>MNSQQNPDLAVHPLAIPMEGLLGESATTLEKNVIATQLSEEAQVKLEVIQSLLEPCDRTTYGQKLREAAEKLNVSLRTVQRLVKNWEQDGLVGLTQTSRADKGKHRIGEFWENFITKTYKEGNKGSKRMTPKQVALRVEAKARELKDSKPPNYKTVLRVLAPILEKQQKAKSIRSPGWRGTTLSVKTREGKDLSVDYSNHVWQCDHTRVDVLLVDQHGEILSRPWLTTVIDTYSRCIMGINLGFDAPSSGVVALALRHAILPKRYGSEYKLHCEWGTYGKPEHFYTDGGKDFRSNHLSQIGAQLGFVCHLRDRPSEGGVVERPFKTLNDQLFSTLPGYTGSNVQERPEDAEKDARLTLRELEQLLVRYIVDRYNQSIDARMGDQTRFERWEAGLPTVPVPIPERDLDICLMKQSRRTVQRGGCLQFQNLMYRGEYLAGYAGETVNLRFDPRDITTILVYRQENNQEVFLTRAHAQGLETEQLALDEAEAASRRLRTAGKTISNQSLLQEVVDRDALVATKKSRKERQKLEQTVLRSAAVDESNRESLPSQIVEPDEVESTETVHSQYEDIEVWDYEQLREEYGFGSEFELENLYFQ[4x]

CRISPR-associated transposons (CASTs) are mobile genetic elements that co-opted CRISPR-Cas systems for RNA-guided transposition. TnsB transposases belong to the retroviral integrase superfamily with an RNase H fold catalytic domain and a DDE active site motif. TnsB associates with the left and right ends of the transposon and catalyses their cleavage generating free 3′-hydroxyl groups, which are later used in a nucleophilic attack downstream of the target sequence. Finally, it performs the strand-transfer reaction that leads to the insertion of the DNA cargo into the target site.

To comprehend how shTnsB facilitates RNA-guided transposition in the CAST V-K system, we determine the structure of the shTnsB-DNA complex captured after the strand-transfer reaction by single-particle cryo-EM at 2.46 Å resolution. The structure reveals an entangled architecture of the shTnsB protein around the DNA building a pseudo-symmetrical assembly in which the four subunits of shTnsB can be grouped in two different conformations. The protein is found in two different conformations to associate with the STC DNA and build the complex. shTnsB1 and 2 depict an extended conformation along the branched nucleic acid structure, where we could not observe the OD and CTD domains. In both protomers, each of the NTD1 and NTD2 domains is associated with LTR(8) and LTR(6), while the catalytic DDE domain is visualized in trans at the junction between the target DNA and the transposon ends. Thus, shTnsB1 accomplishes DNA recognition in the LTR(8) end, and its DDE domain catalyses the attack of the 3´OH in the LTR(6) branch on the target DNA, promoting the strand-transfer reaction. The shTnsB3 and 4 protomers are arranged in a different conformation with few contacts with the backbone of the DNA. The DDE pockets of shTnsB3 and 4 do not contact the DNA and the catalytic residues of these subunits are not properly positioned for the cleavage reaction. In shTnsB the DDE motif consists of two aspartic acid residues (D205, D287) and a glutamic acid (E321) residue, located in a conserved core that forms a characteristic RNase H-like fold combining α-helices and β-strands. E321 is 6 Å away, as the structure is captured in the post-catalytic state. The distances of the extra density to D205, D287 and the backbone phosphates suggest that the density could be assigned to the H2O molecule generated after the 3′-OH attack of one of the strands of the transposable element to the target DNA.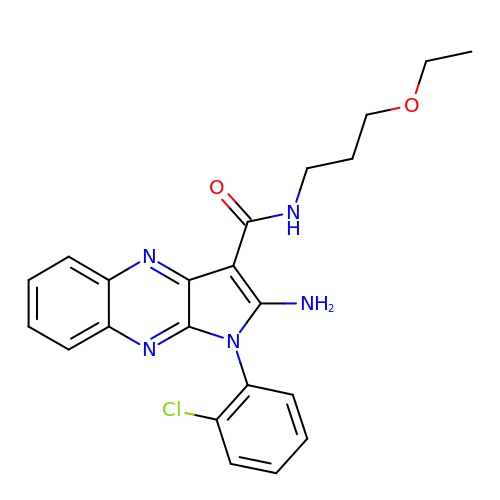2-amino-1-(2-chlorophenyl)-N-(3-ethoxypropyl)-1H-pyrrolo[2,3-b]quinoxaline-3-carboxamide | C22 H22 Cl N5 O2 | JFHMDUNXLJNQOU-UHFFFAOYSA-N> SHDQHAV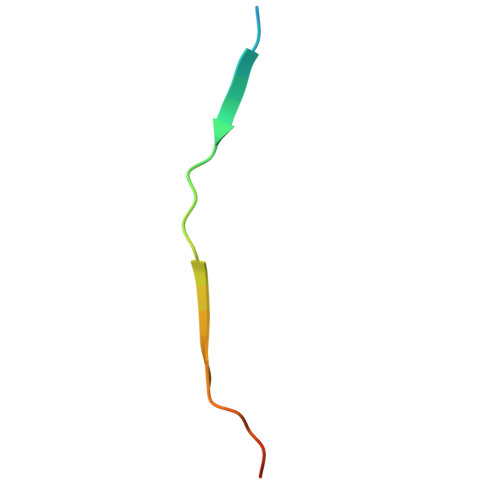LVLQPAVEAFFLVHATERESK> GSHMKNSVSVDLPGSMKVLVSKSSNADGKYDLIATVDALELSGTSDKNNGSGVLEGVKADASKVKLTISDDLGQTTLEVFKSDGSTLVSKKVTRADGTRLEYTGIKSDGSGKAKEVLKGYVLEGTLTAEKTTLVVKEGTVTLSKNISKSGE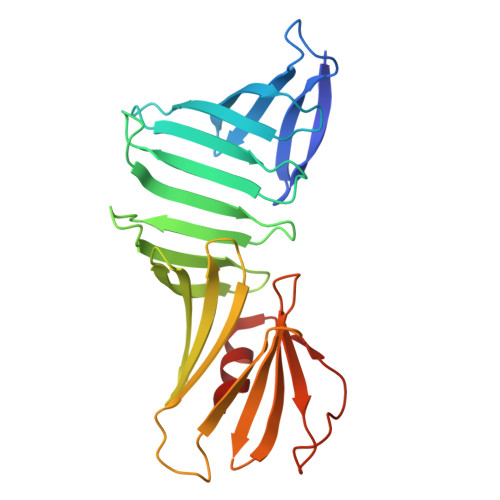VSVELNDTDSSAATKKTAAWNSGTSTLTITVNSKKTKDLVFTSSNTITVQQYDSNGTSLEGSAVEITKLDEIKNALK> QLTPTFYDNSCPNVSNIVRDTIVNELRSDPRIAASILRLHFHDCFVNGCDASILLDNTTS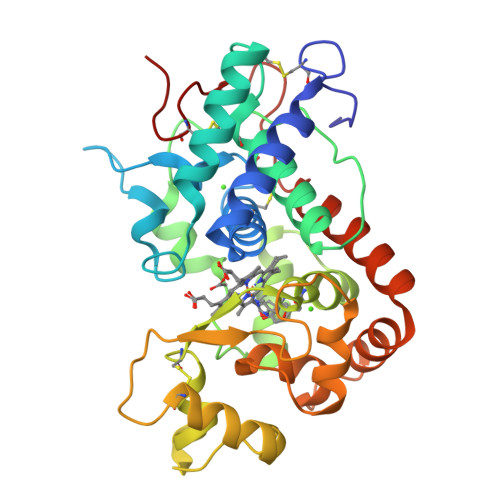FRTEKDAFGNANSARGFPVIDRMKAAVESACPRTVSCADLLTIAAQQSVTLAGGPSWRVPLGRRDSLQAFLDLANANLPAPFFTLPQLKDSFRNVGLNRSSDLVALYGGHTFGKNQCRFIMDRLYNFSNTGLPDPTLNTTYLQTLRGLCPLNGNLSALVDFDLRTPTIFDNKYYVNLEEQKGLIQSDQELFSSPNATDTIPLVRSFANSTQTFFNAFVEAMDRMGNITPLTGTQGQIRLNCRVVNS>YPPSMDWRKKGNFVSPVKNQGSCGSCWTFSTTGALESAVAIATGKMLSLAEQQLVDCAQNFNNHGCQGGLPSQAFEYIRYNKGIMGEDTYPYKGQDDHCKFQPDKAIAFVKDVANITMNDEEAMVEAVALYNPVSFAFEVTNDFLMYRKGIYSSTSCHKTPDKVNHAVLAVGYGEENGIPYWIVKNSWGPQWGMNGYFLIERGKNMCGLAACASYPIPLV[4x];>MIPGGLSEAKPATPEIQEIVDKVKPQLEEKTNETYGKLEAVQYKTQVVAGTNYYIKVRAGDNKYMHLKVFKSLPGQNE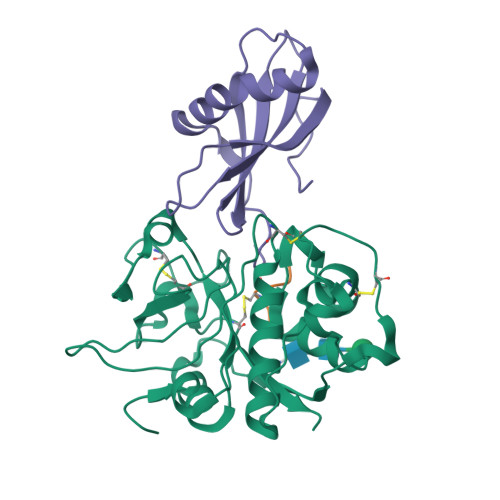DLVLTGYQVDKNKDDELTGF[4x];>[4x]EPQNCSAT>GHMRNVMLITGASRGIGAATALLAAERGYAVVLNYLRNREAAEALRQRIERQGGEALAVAADVAEEGDVERLFASIDERFGRLDVLVNNAGMLEAQTRLENIDAARLHRVFATNVTGSFLCAREAVKRLSTRHGGRGGSIVNVSSMASRLGSPNEYIDYAAAKGAIDSMTIGLAREVAAEGIRVNAVRPGLIDTEIHASGGEPGRIERL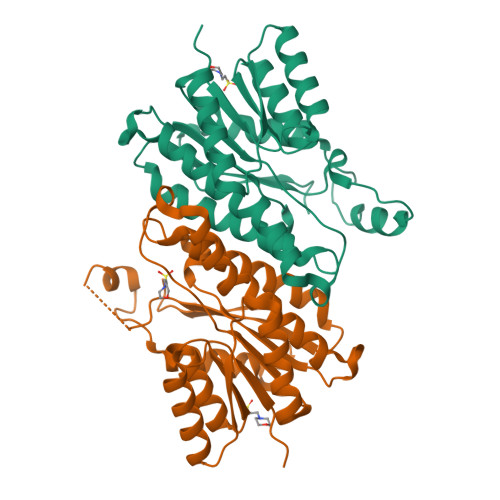KGGIPLGRGGTAEEVARAILWLASDEASYSTGTFIDVSGGR[4x]> GMGEKLELRLKSPVG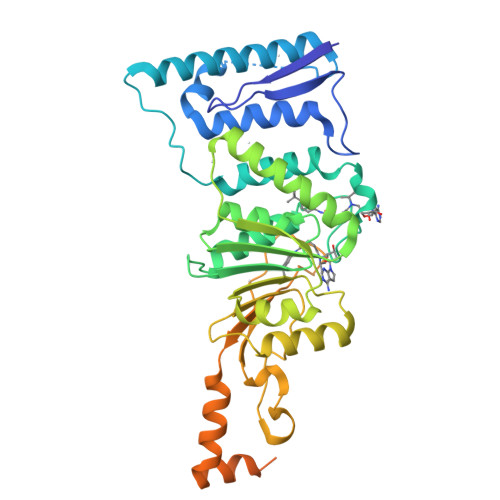AEPAVYPWPLPVYDKHHDAAHEIIETIRWVCEEIPDLKLAMENYVLIDYDTKSFESMQRLCDKYNRAIDSIHQLWKGTTQPMKLNTRPSTGLLRHILQQVYNHSVTDPEKLNNYEPFSPEVYGETSFDLVAQMIDEIKMTDDDLFVDLGSGVGQVVLQVAAATNCKHHYGVEKADIPAKYAETMDREFRKWMKWYGKKHAEYTLERGDFLSEEWRERIANTSVIFVNNFAFGPEVDHQLKERFANMKEGGRIVSSKPFAPLNFRINSRNLSDIGTIMRVVELSPLKGSVSWTGKPVSYYLHTIDRTILENYFSSLKNPKLREEQEAARRRQQRESKSNAATPTKGPEGKVAGPADAPMDSGAEEEKAGAATVKKPSPSKARKKKLNKKGRKMAGRKRG>[2x]EPGRRGSFVEMVDNLRGKSGQGYYVEMTVGSPPQTLNILVDTGSSNFAVGAAPHPFLHRYYQRQLSSTYRDLRKGVYVPYTQGKWEGELGTDLVSIPHGPNVTVRANIAAITESDKFFINGSNWEGILGLAYAEIARPDDSLEPFFDSLVKQTHVPNLFSLQLCGAGFPLNQSEVLASVGGSMIIGGIDHSLYTGSLWYTPIRREWYYEVIIVRV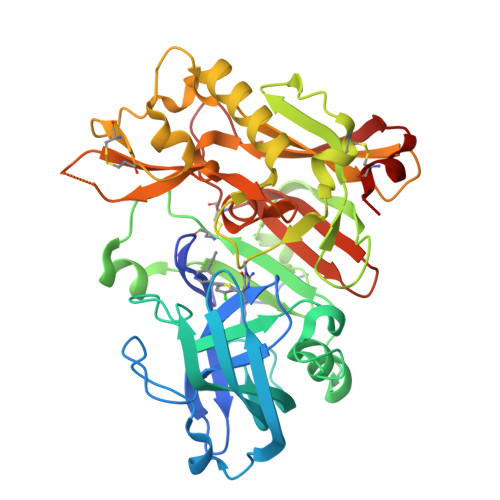EINGQDLKMDCKEYNYDKSIVDSGTTNLRLPKKVFEAAVKSIKAASSTEKFPDGFWLGEQLVCWQAGTTPWNIFPVISLYLMGEVTNQSFRITILPQQYLRPVEDVATSQDDCYKFAISQSSTGTVMGAVIMEGFYVVFDRARKRIGFAVSACHVHDEFRTAAVEGPFVTLDMEDCGYNI>[3x]MPLGLLWLGLALLGALHAQAQDSTSDLIPAPPLSKVPLQQNFQDNQFQGKWYVVGLAGNA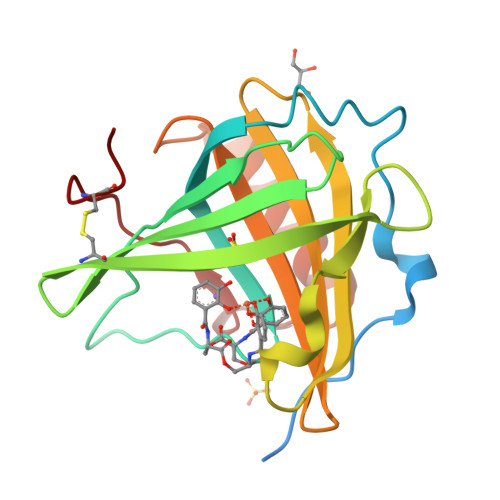ILREDKDPQKMYATIYELKEDKSYNVTSVLFRKKKCDYWIRTFVPGSQPGEFTLGNIKSYPGLTSYLVRVVSTNYNQHAMVFFKAVSQNREYFKITLYGRTKELTSELKENFIRFSKSLGLPENHIVFPVPIDQCIDG> MKKGTASEEELKKLYDPNTFYEHGDNPAFKQFMNIAVENLREGKLTDHRTYVVDTYKKWMYARNWDDFLQRDCKAITFPRAFALWIVGTLGMATASKWCRQIL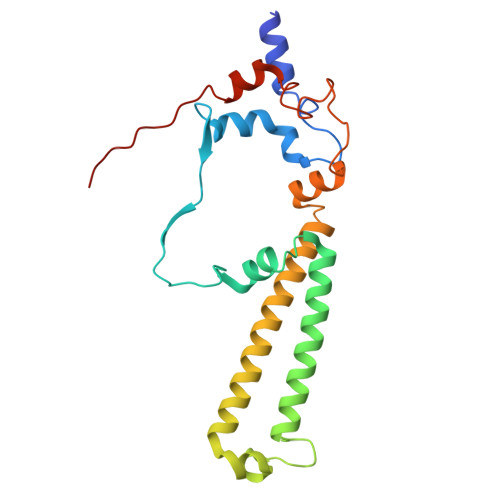PVGSHGITKISQTQFFHQFGPLGTLGAVGFYGLTAYLYYKTTIFTVKKFYSHCILQEREWIFEQERQNPGYGEYFFKDVPLSAEEHFNDLARGEMAKKKFEKPNHEF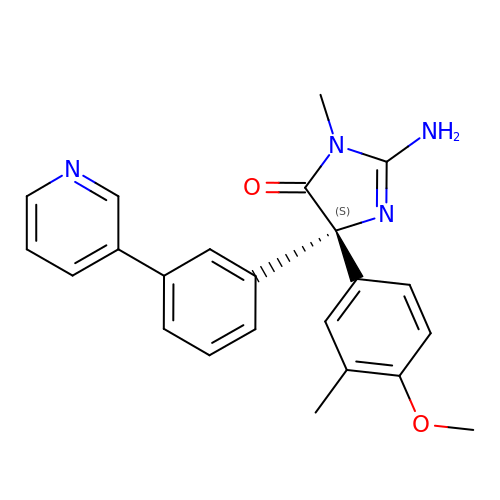(5S)-2-amino-5-(4-methoxy-3-methylphenyl)-3-methyl-5-(3-pyridin-3-ylphenyl)-3,5-dihydro-4H-imidazol-4-one | C23 H22 N4 O2 | TWVGNKMRZLBNOD-QHCPKHFHSA-N>LPSGSDPAFSQPKSVLDAGLTCQGASPSSVSKPILLVPGTGTTGPQSFDSNWIPLSTQLGYTPCWISPPPFMLNDTQVNTEYMVNAITALYAGSGNNKLPVLTWSQGGLVAQWGLTFFPSIRSKVDRLMAFAPDYKGTVLAGPLDALAVSAPSVWQQTTGSALTTALRNAGGLTQIVPTTNLYSATDEIVQPQVSNSPLDSSYLFNGKNVQAQAVCGPLFVIDHAGSLTSQFSYVVGRSALRSTTGQARSADYGITDCNPLPANDLTPEQKVAAAALLAPAAAAIVAGPKQNCEPDLMPYARPFAVGKRTCSGIVTP[2x]

Lipases (EC 3.1.1.3) are ubiquitous hydrolases for the carboxyl ester bond of water-insoluble substrates such as triacylglycerols, phospholipids, and other insoluble substrates, acting in aqueous as well as in low-water media. Among lipases, Candida antarctica lipase B (CALB) is the one that found the widest application in many industrial processes because of its high enantioselectivity, wide range of substrates, thermal stability, and stability in organic solvents. CALB belongs to the α/β hydrolase fold family with a conserved catalytic triad consisting of Ser, His, and Asp/Glu within an acyl binding pocket and a binding pocket for the moiety of secondary alcohols. CALB has two α-helixes surrounding the active site, namely α5 and α10 (14, 15), which have been shown to be very flexible regions and could work as a lipase lid by a relative motion between them either by increasing the working temperature or by working in organic solvents.

Pressurizing the crystal with xenon probed the tightness of the closed lipase conformation. Three xenon atoms, with anomalous signal bigger than 4σ, were located in monomer A in the catalytic site in close proximity to the catalytic triad. In particular, the three xenon atoms (8.3σ, 6.3σ, and 6σ map level, respectively, refined with fractional occupancies) in monomer A are located above His224, in the hydrophobic region of the catalytic site defined by Leu144, Val154, Ile189, Leu219, Val221, Ala281, Ala282, Ile285, and Leu287. No xenon atoms were observed in the active site of monomer B, thus confirming that the conformational rearrangement of the residue range 140–147 prevents the access of any substrate to the active site. Xenon is also found in the hydrophobic cavity defined by Met83, Val101, Leu115, Ile121, Val125, Val37, and Ile187 in both monomer A (10.2σ) and monomer B (10.5σ). A further site is found next to Trp155 in monomer B (7.2σ). The location of three xenon atoms in monomer A, in close proximity to the catalytic triad, and none in monomer B, confirms that the conformational rearrangement of α-helix 5 seals the active site. The unfolding of α-helix 5 results in the closing of the lid over the cavity, preventing the access of any substrate to the catalytic site, as shown by probing binding sites with xenon. Probing the crystals using xenon validated the open and closed conformations.>[4x]GSMTLTAPSKKSTYAPLELFDTDRLLDQDERDIAATVRQFVDTRLKPNVEGWFESATLPSELAKEFGNLGVL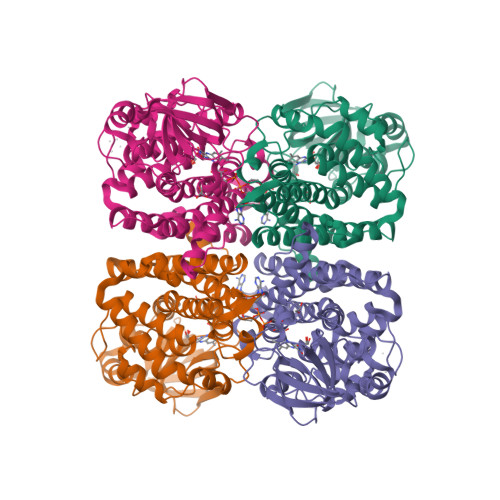GMHLQGYGCAGTNAVSYGLACMELEAGDSGFRSFVSVQGSLSMFSIYRYGSEEQKNEWLPRLAAGDAIGCFGLTEPDFGSNPAGMRTRARRDGSDWILNGTKMWITNGNLADVATVWAQTDDGIRGFLVPTDTPGFTANEIHRKLSLRASVTSELVLDNVRLPASAQLPLAEGLSAPLSCLNEARFGIVFGALGAARDSLETTIAYTQSREVFDKPLSNYQLTQEKLANMTVELGKGMLLAIHLGRIKDAEGVRPEQISLGKLNNVREAIAIARECRTLLGGSGITLEYSPLRHANNLESVLTYEGTSEMHLLSIGKALTGKAAFRS> FTLIELMIVIAIVGILAAVALPAYQDYTARAQVSEAILLAEGQKSAVTEYYLNHGKWPENNTSAGVASSPTDIKGKYVKEVEVKNGVVTATMLSSGVNNEIKGKKLSLWARRENGSVKWFCGQPVTRTDDDTV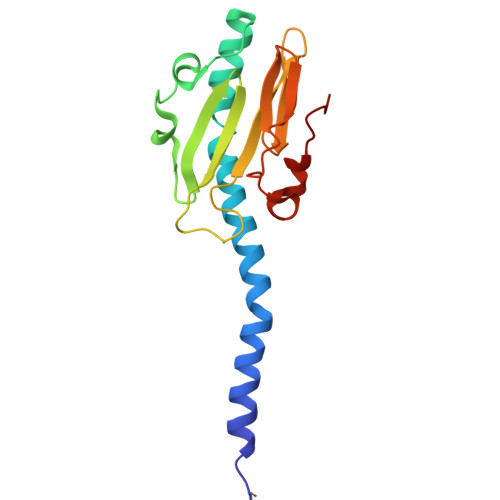ADAKDGKEIDTKHLPSTCRDNFDAK>MRGSHHHHHHGSAEPPNMPSMAPVLKNIMPAIVNVAVQGYLPNDVTPPGSAGNDEENQPNNRPPQSRMPEKGRKFESIGSGVIIDPNNGVIITNDHVIRNASLITVTLQDGRRLKARLIGGDSETDLAVLKIDAKNLKSLVIGD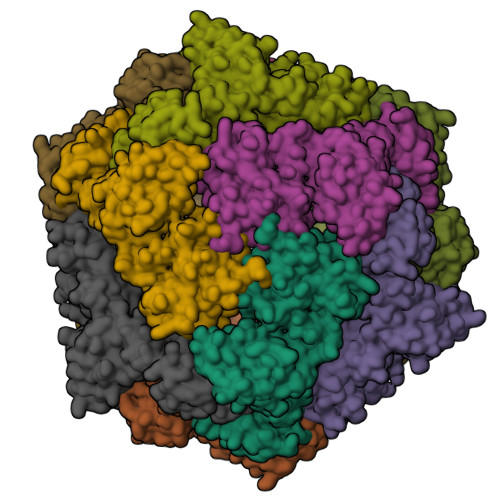SDKLEVGDFVVAIGNPFGLNSFGNSQSATFGIVSALKRSDLNIEGVENFIQTDAAINPGNSGGALVNAKGELIGINTAILSPYGGNVGIGFAIPINMVKDVAQQIIKFGSIHRGLMGIFVQHLTPELAQAMGYPEDFQGALVSQVNPNSPAELAGLKAGDIITQINDTKITQATQVKTTISLLRVGSTVKIIVERDNKPLTLSAVVTDIKSHEQKLQSNNPFLYGLALRAFEQESPPHGNVIGVQVVGASENSAGWRAGIRPGDIIISANKKPVTDVKSLQTIAQEKKKELLVQVLRGPGSMYLLVI[4x]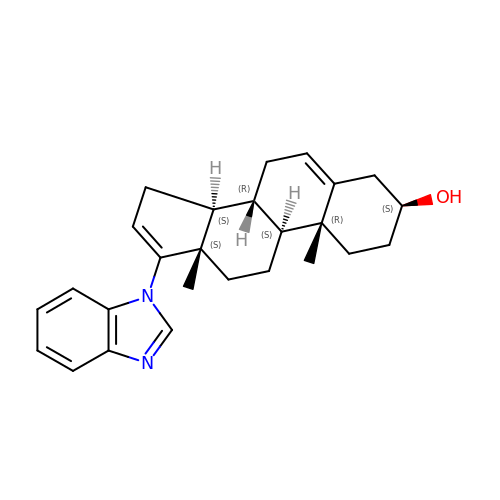(3alpha,8alpha)-17-(1H-benzimidazol-1-yl)androsta-5,16-dien-3-ol | C26 H32 N2 O | PAFKTGFSEFKSQG-PAASFTFBSA-N> GGSGSMALIMEPVSKWSPSQVVDWMKGLDDCLQQYIKNFEREKISGDQLLRITHQELEDLGVSRIGHQELILEAVDLLCALNYGLETENLKTLSHKLNASAKNLQNFITGRRRSGHYDGRTSRKLPNDFLTSVVDLIGAAKSLLAWLDRSPFAAVTDYSVTRNNVIQLCLELTTIVQQDCTVYETENKILHVCKTLSGVCDHIISLSSDPLVSQSAHLEVIQLANIKPSEGLGMYIKSTYDGLHVITGTTENSPADRCKKIHAGDEVIQVNHQTVVGWQLKNLVNALREDPSGVILTLKKRPQSMLTSAPALLKNMRWK;> GPGSTQQDVCKWLKKHCPNQYQLYSESFKQHDITGRALLRLTDKKL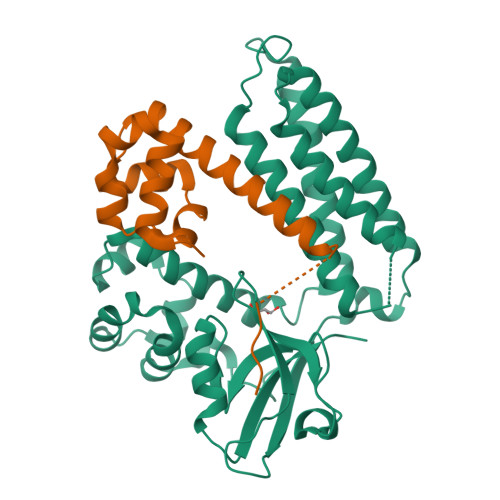ERMGIAQENQRQHILQQVLQLKVREEVRNLQLLTQASVECSPGSGSENLYFQ>[2x]GAMNQSASEQLQTDIP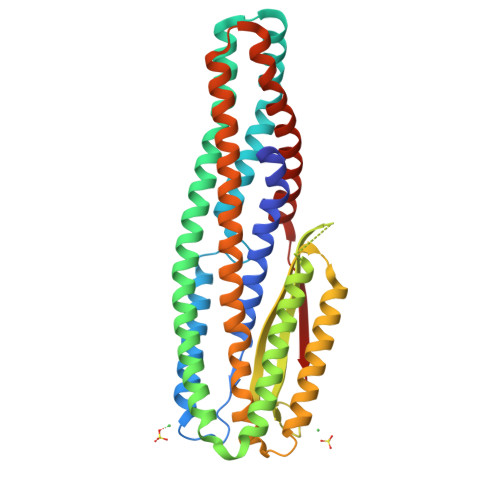ASISAMVLLNSACQGVVETYIDQGNAEHWYAQVEQNLNAVQKLVRQWRLSGNLYFSNDIMDSVLSIANTFKDSNVQILTLFKALETRFDTAQLQQLTSLILTLQNPIQSLTSNIKRYDEGLNAWARQVEDAHNTLQQTIAQIQQEEVSIQAEIIATNAQIDLMKQQIAAFKTAIANAQSQRKKGIFETIFGVVLAPFTLGGSLILAGFGVSSIVEAQSEISSLQSDIQSSLNTINHDQQTLSQDQQQIASLNALLLSVDQVNNDCAAISRSLDTLQTTVLSLYNETNNVVSNLTKAQDSQAVILEQVWYQSAYNEWQDILEVASTLNNAQPQITKAQIK>GPGSEFDTRHETREDRTKRLFRHYTVGSYDSLTSHSDYVIDDKVAILQKRDHEGFGFVLRGAKAETPIEEFTPTPAFPALQYLESVDVEGVAWRAGLRTGDFLIEVNGVNVVKVGHKQVVGLIRQGGNRLVMKVVSVTR[2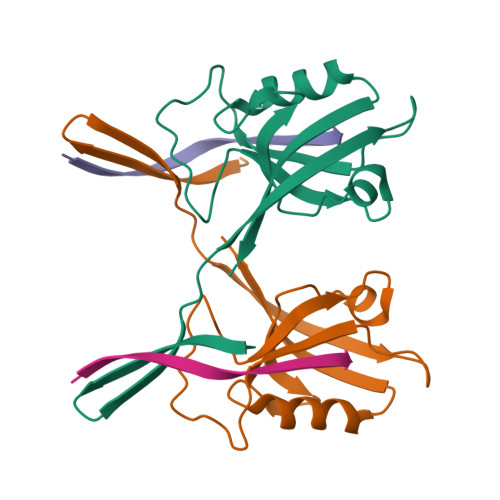x];>[2x]ADSIEIYIPEAQTRL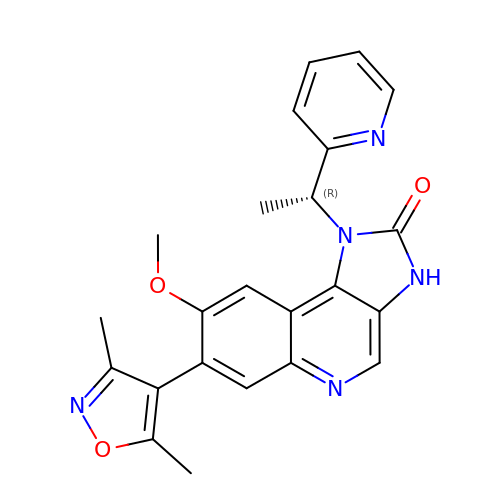7-(3,5-DIMETHYL-1,2-OXAZOL-4-YL)-8-METHOXY-1-[(1R)-1-(PYRIDIN-2-YL)ETHYL]-1H,2H,3H-IMIDAZO[4,5-C]QUINOLIN-2-ONE | C23 H21 N5 O3 | VUVUVNZRUGEAHB-CYBMUJFWSA-N> MAAGKLKKEQQNQSAERESADTGKVNDEDEEHLYGNIDDYKHLIQDEEYDDEDVPHDLQLSEDEYNSERDSSLLAEFSDYGEISEDDEEDFMNAIREASNFKVKKKKKNDKGKSYGRQRKERVLDPEVAQLLSQANEAFVRNDLQVAERLFNEVIKKDARNFAAYETLGDIYQLQGRLNDCCNSWFLAAHLNASDWEFWKIVAILSADLDHVRQAIYCFSRVISLNPMEWESIYRRSMLYKKTGQLARALDGFQRLYMYNPYDANILRELAILYVDYDRIEDSIELYMKVFNANVERREAILAALENALDSSDEESAAEGEDADEKEPLEQDEDRQMFPDINWKKIDAKYKCIPFDWSSLNILAELFLKLAVSEVDGIKTIKKCARWIQRRESQTFWDHVPDDSEFDNRRFKNSTFDSLLAA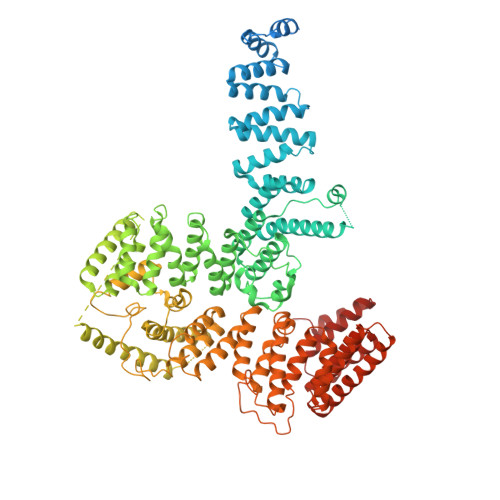EKEKSYNIPIDIRVRLGLLRLNTDNLVEALNHFQCLYDETFSDVADLYFEAATALTRAEKYKEAIDFFTPLLSLEEWRTTDVFKPLARCYKEIESYETAKEFYELAIKSEPDDLDIRVSLAEVYYRLNDPETFKHMLVDVVEMRKHQVDETLHRISNEKSSNDTSDISSKPLLEDSKFRTFRKKKRTPYDAERERIERERRITAKVVDKYEKMKKFELNSGLNEAKQASIWINTVSELVDIFSSVKNFFMKSRSRKFVGILRRTKKFNTELDFQIERLSKLAEGDSVFEGPLMEERVTLTSATELRGLSYEQWFELFMELSLVIAKYQSVEDGLSVVETAQEVNVFFQDPERVKMMKFVKLAIVLQMDDEEELAENLRGLLNQFQFNRKVLQVFMYSLCRGPSSLNILSSTIQQKFFLRQLKAFDSCRYNTEVNGQASITNKEVYNPNKKSSPYLYYIYAVLLYSSRGFLSALQYLTRLEEDIPDDPMVNLLMGLSHIHRAMQRLTAQRHFQIFHGLRYLYRYHKIRKSLYTDLEKQEADYNLGRAFHLIGLVSIAIEYYNRVLENYDDGKLKKHAAYNSIIIYQQSGNVELADHLMEKYLSIRSGG> STSSAIELLPFHCPFAAAVNPRLAEIEKLCVDWIDEFRLYQDDAQRERLIATKAAEVYARALPNAAPERVADVAKWLYWGFATDDMVYDNGPVSVRAADFLPLIVQLARIADEPRSRFGFEIPYTDALRDLTVAITAPATPGQRIEWRSTARAWFFGMSWDVAYAERGEIPSLNDYLMMRMHTGGLASWAATLGIADGFELSARDADSPAVRALLESWSTFALIINDLMSYAKEIENKDTSSNIITVIARELSCSPQEAVPHAYSILDRISGLFLRLRADLLPGADQNLRALIAGMEHTWRAYL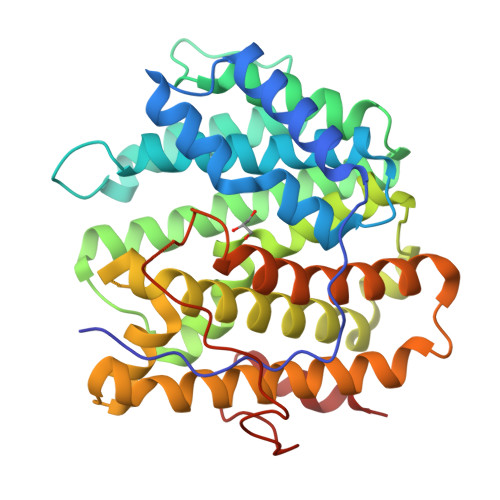DWGFTSARYTRRDPGSEPYQVFPGWAEQPHDTSPDPLPYPAIAWWWEQVAGS>SNAMHMLRIAKEALTFDDVLLVPAHSTVLPNTADLRTRLTKNIALNIPMVSASMDTVTEARLAIALAQEGGIGFIHKNMSIEQQAAQVHQVKISGGLRVGAAVGAAPGNEERVKALVEAGVDVLLIDSSHGHSEGVLQRIRETRAAYPHLEIIGGNVATAEGARALIEAGVSAVKVGIGPGSICTTRIVTGVGVPQITAIADAAGVANEYGIPVIADGGIRFSGDISKAIAAGASCVMVGSMFAGTEEAPGEVILYQGRSYKAYRGMGSLGAMSKGSS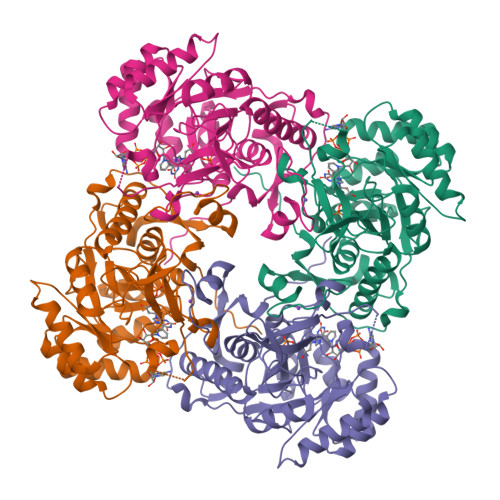DRYFQTDNAADKLVPEGIEGRIAYKGHLKEIIHQQMGGLRSCMGLTGSATVEDLRTKAQFVRISGAGMKESHVHDVQITKEAPNYRLG[2x]>SNAMVAKQ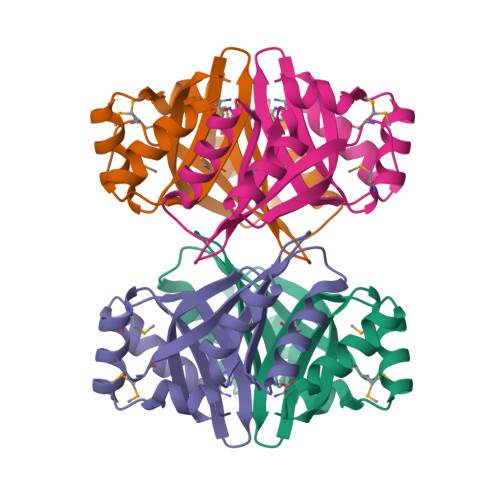LSIFLENKSGRLTEVTEVLAKENINLSALCIAENADFGILRGIVSDPDKAYKALKDNHFAVNITDVVGISCPNVPGALAKVLGFLSAEGVFIEYMYSFANNNVANVVIRPSNMDKCIEVLKEKKVDLLAASDLYKL[2x]> MAKATTSVNYASNLDKRLPELPEGANRAQILESTWSTEFKVYDSFGEAHELQIDFARVPGEVNAWRATVNVDPTNADATATRVGIGTTDGVQNSFIVRFDNNGHLASVTDTAGNVTS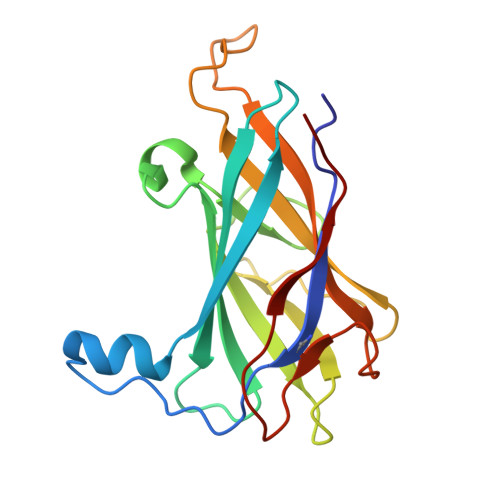PAGQVLVQISYNVVGANPDEAGAPTRHTFDVNLGEIGTSKNTITQFSDKSTTKAYEQDGYT6-(4-fluorophenyl)-8-oxidanyl-3~{H}-quinazolin-4-one 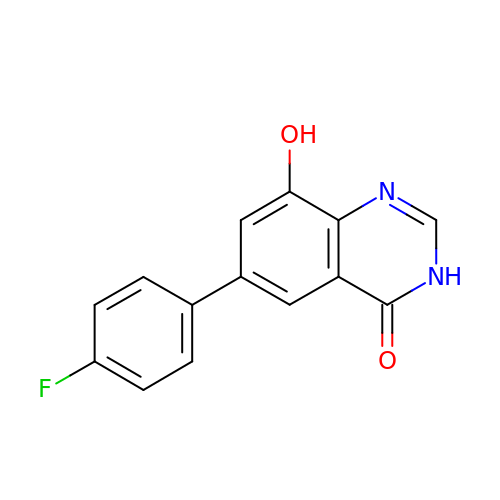| C14 H9 F N2 O2 | MVFBYXBGOWGDLX-UHFFFAOYSA-N cis-4-{[2-(1H-benzimidazol-5-ylamino)quinazolin-8-yl]oxy}cyclohexanol | C21 H21 N5 O2 | 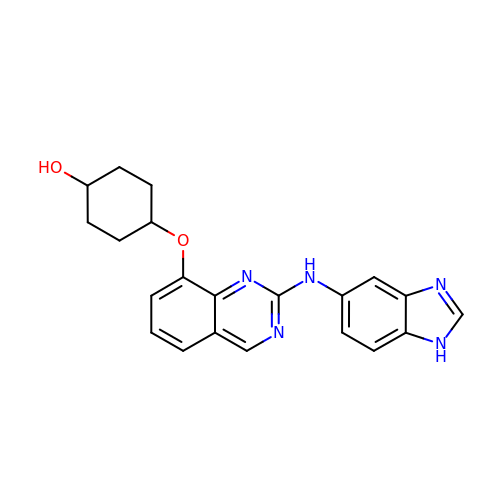FYWRWBSYRGSWIQ-IYBDPMFKSA-N(6P)-4-amino-6-(2H-tetrazol-5-yl)benzene-1,3-disulfonamide | C7 H9 N7 O4 S2 | 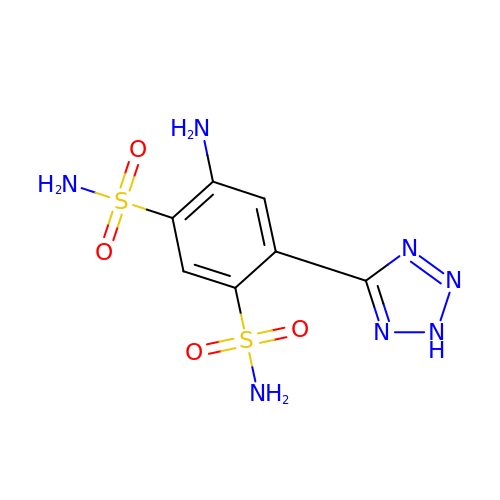HZKIZEMGGDWFAS-UHFFFAOYSA-N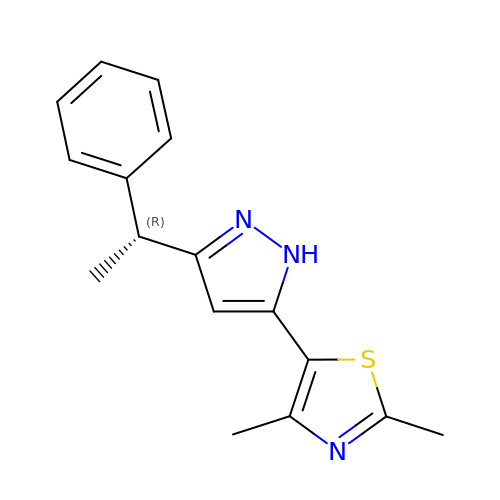2,4-dimethyl-5-{3-[(1R)-1-phenylethyl]-1H-pyrazol-5-yl}-1,3-thiazole | C16 H17 N3 S | BUFWVGVUFJNORA-SNVBAGLBSA-N>MASSCAVQVKLELGHRAQVRKKPTVEGFTHDWMVFVRGPEHSNIQHFVEKVVFHLHE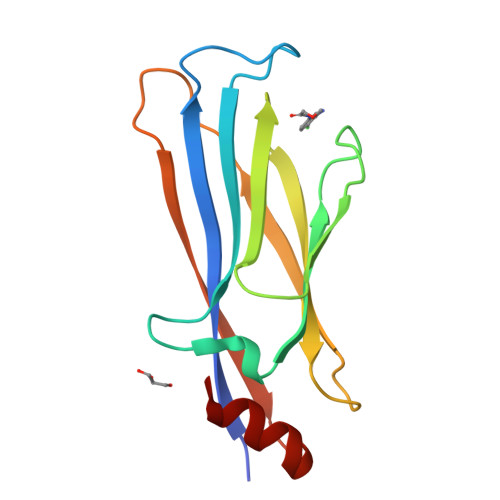SFPRPKRVCKDPPYKVEESGYAGFILPIEVYFKNKEEPRKVRFDYDLFLHLEGHPPVNHLRCEKLTFNNPTEDFRRKLLKA[2x]> MTVSASKTAQQLKYIKDSIKTIPDYPKAGILFRDVTSLLENPKAYSASIELLSEHYSESGVTKVVGTEARGFLFG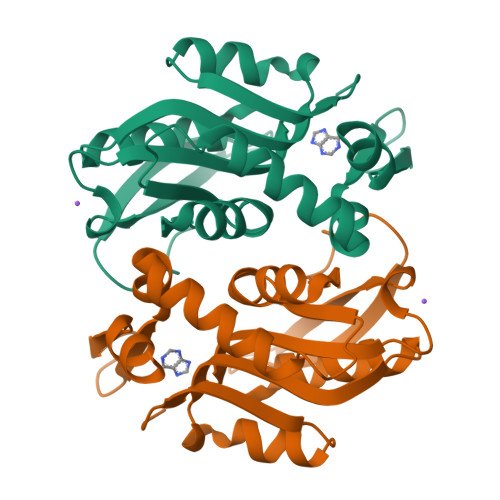APVALALGVGFVPVRKPGKLPRETISESYELEYGTDTLEIHTDSIQPGDKVLVVDDLLATGGTIEATVKLIRRLGGEVVHAAFIINLPELGGEARLTQQGIHCYSLVSFDGH> MSAPTDDTPTDAIAAPRHSAPPRPRLPWFLRTFAVPIILAWVAVVAILNTVVPTLDEVGEMRAVSMAPNDAPSTLAIKRVGQVFEEYDTSSSVMIVLEGEEPLGIEAHAFYDKMVADLRADTEHVQHVQDFWGDTLTASGAQSVDGKAAYVQVYIAGDQGESLANESVEAVRKIATERETPSGVKAYVTGAAATSADQRAEGDASMKLIEGVTFAVITVMLLAVYRSVITTLIVLAMVVLGLSGARGIVAFLGFYNVFGLTTFATNMVVTLAIAAATDYAIFLIGRYQEARRAGEDRESAYYTMFHGTAHVVLASGLTIAGATLCLHFTRLPYFQTMGVPLAIGMLIVVAAALTAGPAVISVVSRFGKTLEPKRFSRSPGWHRVGTATVRWPGAILVCAVVAALIGLLALPGYYTTYDDRRYLPDDVPANVGYDAAFRHFSQAKMNPDLMMVETDRDLRNPADFLVIDKIAKALKNVHGIAQVQTITRPDGDPIEHSTIPYTIGQSGTTQIMNNDYMQTNLDNLLKQADDLQTSIDSMTEMMNIQTELAAVSQSMADKMAQTSDDTADVRDHLADFDDFFRPIRNYLY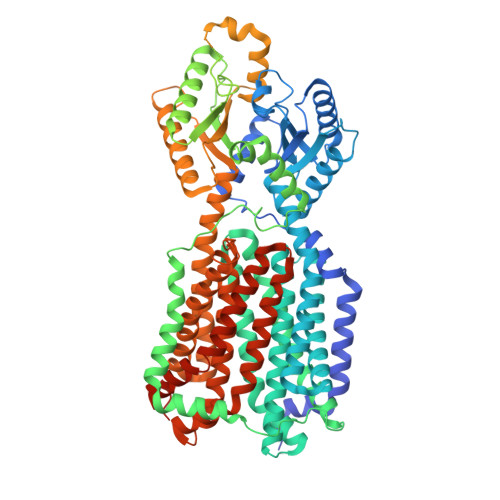WEPHCYDIPMCWSMRSIFESIDGINTMSDDFQELVPEMRRMADLMPRMVAVMPAQIQSMKNQKQTLLNQYQVQKAQQDQNMAMQENATAMSQAFDAAKNDDSFYLPPEAFETDDFQRGMKLFMSPDGHAVRFTIIHQGDPLTEEGTARMDELKVAAADAIKGTPFEGARIYLGGSAATYNDMQIGADYDLIIVAASALILIFIIMMVLTRAVVAAAVIVGTVVLSLASAFGLSVLLWQHIVGIPLHWMVLPMSVIVLLAVGADYNLLLVSRMKEEIHAGIRTGIIRAMVGTGAVVTAAGLVFAFTMASMAVSSLITIGQVGTTIGLGLLFDTLVVRSLMTPSIATLLGRWFWWPQRVRERPVPSKWPTPIQRTPEEALSHHHHHH>GHMASGSMEMEQEKMTMNKELSPDAAAYCCSACHGDETWSYNHPIRGRAKSRSLSASPALGSTKEFRRTRSLHGPCPVTTFGPKACVLQNPQTIMHIQDPASQRLTWNKSPKSVLVIKKMRDASLLQPFKELCTHLMEENMIVYVEKKVLEDPAIASDESFGAVKKKFCTFREDYDDISNQIDFIICLGGDGTLLYASSLFQGSVPPVMAFHLGSLGFLTPFSFENFQSQVTQVIEGNAAVVLRSRLKVRVVKELRGKKTAVHNGLGEN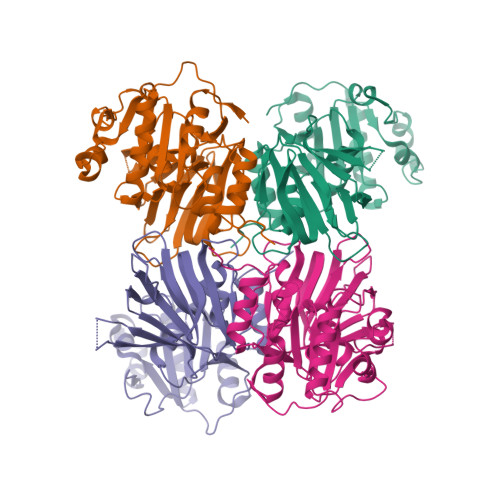GSQAAGLDMDVGKQAMQYQVLNEVVIDRGPSSYLSNVDVYLDGHLITTVQGDGVIVSTPTGSTAYAAAAGASMIHPNVPAIMITPICPHSLSFRPIVVPAGVELKIMLSPEARNTAWVSFDGRKRQEIRHGDSISITTSCYPLPSICVRDPVSDWFESLAQCLHWNVRKKQAHFEEEEEEEEEG[4x]>MKNSKAILQVPGTMKIISAEIPVPKEDEVLIKVEYVGICGSDVHGFESGPFIPPKDPNQEIGLGHECAGTVVAVGSRVRKFKPGDRVNIEPGVPCGHCRYCLEGKYNICPDVDFMATQPNYRGALTHYLCHPESFTYKLPDNMDTMEGTLVEPAAVGMHAAMLADVKPGKKIIILGAGCIGLMTLQACKCLGATEIAVVDVLEKRLAMAEQLGATVVINGAKEDTIARCQQFTEDMGADIVFETAGSAVTVKQAPYLVMRGGKIMIVGTVPGASAINFLKINR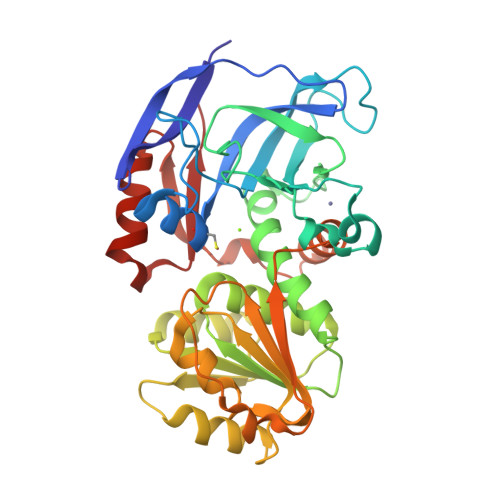EVTIQTVFRYANRYPVTIEAISSGRFDVKSMVTHIYDYRDVQQAFEESVNNKRDIIKGVIKISD[2x]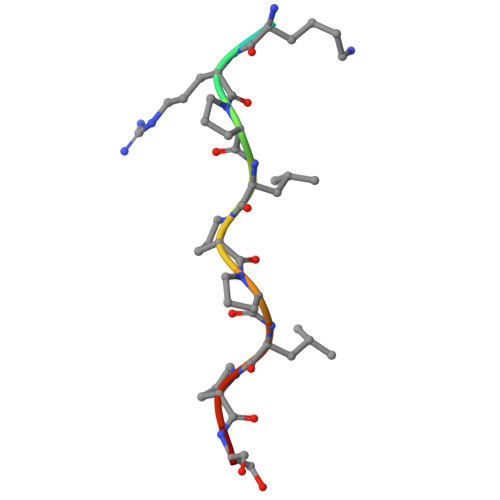> HSKRPLPPLPSL>MTRYDSLLQALGNTPLVGLQRLSPRWDDGRDGPHVRLWAKLEDRNPTGSIKDRPAVRMIEQAEADGLLRPGATILEPTSGNTGISLAMAARLKGYRLICVMPENTSVERRQLLELYGAQIIFSAAEGGSNTAVATAKELAATNPSWVMLYQYGNPANTDSHYCGTGPELLADLPEITHFVAGLGTTGTLMGTGRFLREHVANVAIVAAEPRYGEGVYALRNMDEGFVPELYDPEILTARYSVGAVDAVRRTRELVHTEGIFAGISTGAVLHAALGVGAGALAAGERADIALVVA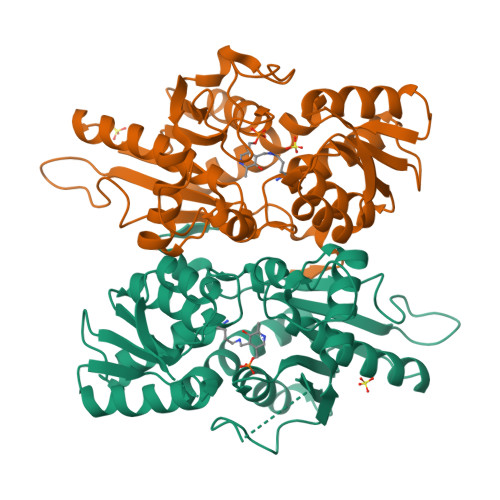DAGWKYLSTGAYAGSLDDAETALEGQLWA[2x]>[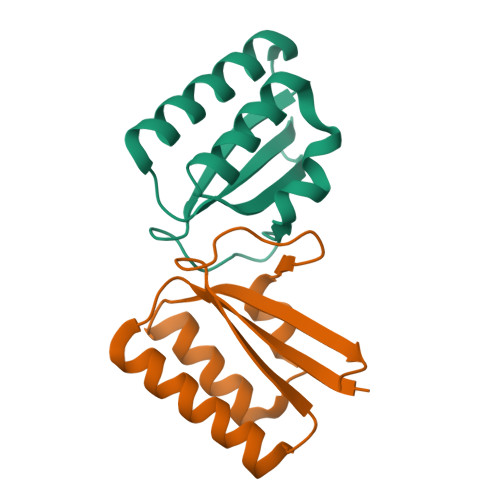2x]MNKARKTYVLKLYVAGNTPNSVRALKTLKNILEQEFQGIYALKVIDVLKNPQLAEEDKILATPTLSKILPPPVRKIIGDLSDRERVLIGLDLLYEELTEEDWEAQSNL> MRERPHTSGHHGAGEARATAPSTVSPYGPEARAELSSRLTTLRNTLAPATNDPRYLQACGGEKLNRFRDIQCRRQTAVRADLNANY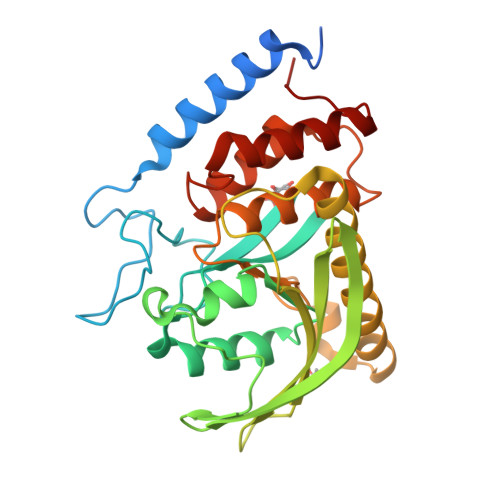IQVGNTRTIACQYPLQSQLESHFRMLAENRTPVLAVLASSSEIANQRFGMPDYFRQSGTYGSITVESKMTQQVGLGDGIMADMYTLTIREAGQKTISVPVVHVGNHPDQTAVSSEVTKALASLVDQTAETKRNMYESKGSSAVADDSKLRPVIHCRAGVGRTAQLIGAMCMNDSRNSQLSVEDMVSQMRVQRNGIMVQKDEQLDVLIKLAEGQGRPLLNS>MGHHHHHHHHHHSSGHIEGRHMFSKLHATPPQTVAVAPSGAAEIASERLEPRVEEKDGYWVLKEKFRQGINPAEKAKIEKEPMKLFMENGIEDLAKISLEEIEGSKLTKDDIDVRLKWLGLFHRRKHHYGRFMMRLKLPNGVTTSSQTRYLASVIRKYGKDGCADVTTRQNWQIRGVVLPDVPEILKGLDEVGLTSLQSGMDNVRNPVGNPLAGIDPHEIVDTRPYTNLLSQYVTANFRGNPAVTNLPRKWNVCVIGSHDLYEHPQINDLAYMPATKDGRFGFNLLVGGFFSPKRCAEAVPLDAWVPADDVVPVCKAILEAYRDLGTRGNRQKTRMMWLVDELGVEGFRAEVVKRMPQQKLDRESTEDLVQKQWERREYLGVHPQKQEGYSFVGLHIPVGRVQADDMDELARLADEYGSGELRLTVEQNIIIPNVKNSKIEALLNEPLLKNRFSTDPPILMKNLVACTGNQFCGKAIIETKARSMKITEEVQLLVSITQPVRMHWTGCPNSCAQVQVADIGFMGCLTRKEGKTVEGADVYLGGRIGSDS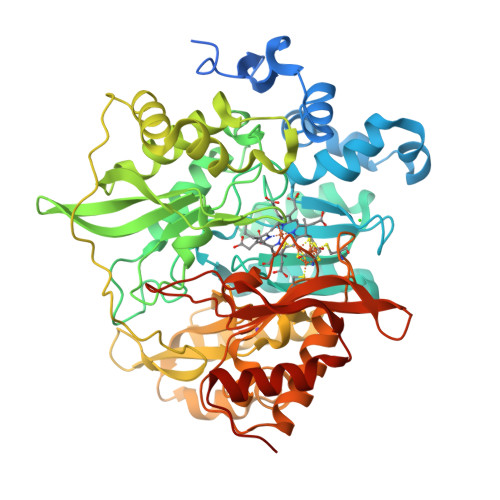HLGDVYKKSVPCEDLVPIIVDLLVDNFGAVPREREEAED[2x]> FSAQTNRHILRFNRPFLVVIFSTSTQSVLFLGKVVDP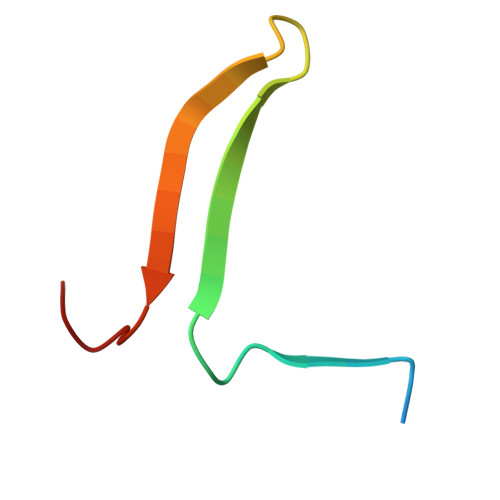TKP> ANVRLQHHHHHHHENLYFQGLEYQFEVQGQSEYVDTTANDKNFTGTAQGTYYFKNVDASKGPLAEAAFLNQASNVSVAYNYIKYDEKDTVNVESHTYGVKGEAYLPTPYLP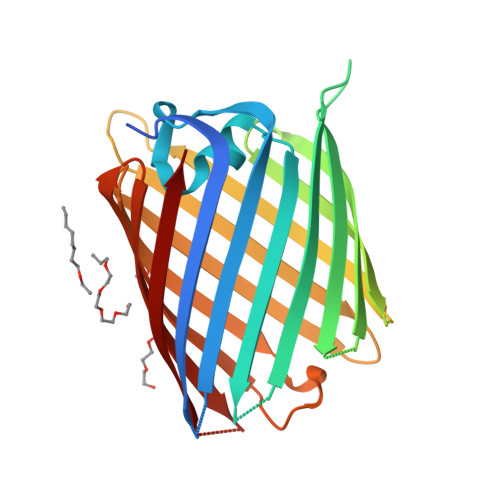VYASASYNHTINDFKDGVSDDNGDRYALEAGAMLLPNFLVAVGYTSVADQISLDAFGVNKYGIAKAVGESVAIDEKQDAVTARTKYVGNIDGTNMAIGFEAFGVFAEDNAYGMKTDLFVTPKLSVGASFADVSAFNSGYDHVWGGHTQYFITPAVAVGADFVKANAKDGNPRDTQTIGLNAKFRF> DLLSCLTFNGVRNHTVFSADSDSDFNRFLHLSIQNPLFQNSLISKPSAIILPGSKEELSNTIRCIRKGSWTIRLRSGGHSYEGLSYTSDTPFILIDLMNLNRVSIDLESETAWVESGSTLGELYYAITESSSKLGFTAGWAPTVGTGGHISGGGFGMMSRKYGLAADNVVDAILIDANGAILDRQAMGEDVFWAIRGGGGGVWGAIYAWKIKLLPVPEKVTVFRVTKNVAIDEATSLLHKWQFVAEELEEDFTLSVLGGADEKQVWLTMLGFHFGLKT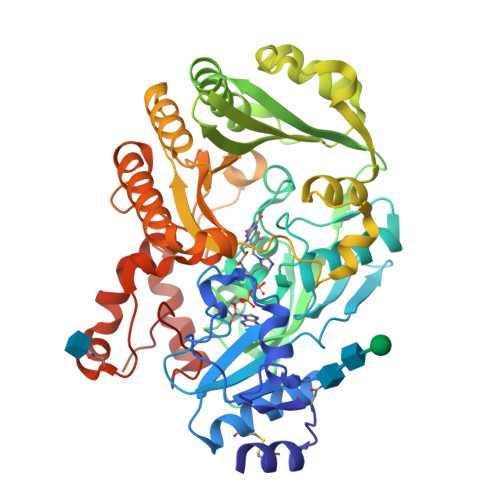VAKSTFDLLFPELGLVEEDYLEMSWGESFAYLAGLETVSQLNNRFLKFDERAFKTKVDLTKEPLPSKAFYGLLERLSKEPNGFIALNGFGGQMSKISSDFTPFPHRSGTRLMVEYIVAWNQSEQKKKTEFLDWLEKVYEFMKPFVSKNPRLGYVNHIDLDLGGIDWGNKTVVNNAIEISRSWGESYFLSNYERLIRAKTLIDPNNVFNHPQSIPPMA>SNAMADEIAKAQVARPGGDTIFGKIIRKEIPAKIIFEDDRCLAFHDISPQAPTHFLVI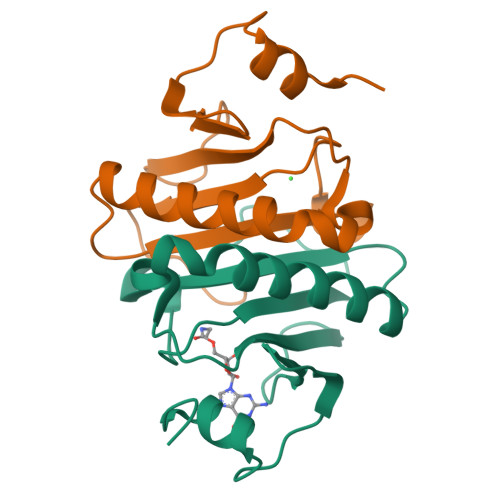PKKHISQISVAEDDDESLLGHLMIVGKKCAADLGLNKGYRMVVNEGSDGGQSVYHVHLHVLGGRQMHWPPG[2x]>MSIAESSVPIAVPVPTGGDDPTKVAMLGLTFDDVLLLPAASDVVPATADTSSQLTKRIRLRVPLVSSAMDTVTESRMAIAMARAGGMGVLHRNLPVAEQAGQVETVKRSEAGMVTDPVTCSPDNTLAEVDAMCARFRISGLPVVDDTGELVGIITNRDMRFEVDQSKPVSEVMTKAPLITAKEGVSAEAALGLLRRHKIEKLPIVDGHGKLTGLITVKDFVKTEQFPLSTKDSDGRLLVGAAVGVGDDAWTRAMTLVDAGVDVLIVDTAHAHNRGVLDMVSRLKQAVGERVDVVGGNVATRAAAAALVEAGADAVKVGVGPGSICTTRVVAGVGAPQITAILEAVAACKPYGVPVIADGGLQYSGD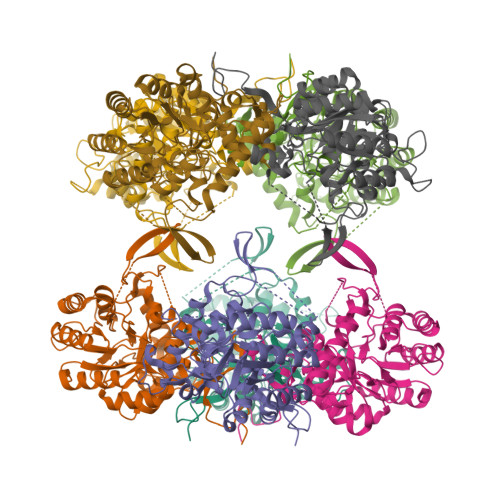IAKALAAGASTAMLGSLLAGTAESPGELIFVNGKQFKSYRGMGSLGAMQGRGAAKSYSKDRYFQDDVLSEDKLVPEGIEGRVPFRGPLGTVIHQLTGGLRAAMGYTGSATIEQLQQAQFVQITAAGLKESHPHDITMTVEAPNYYTR[8x]> MGSSHHHHHHSSPISPIETVPVKLKPGMDGPKVKQWPLTEEKIKALVEICTEMEKEGKISKIGPENPYNTPVFAIKKKDSTKWRKLVDFRELNKRTQDFWEVQLGIPHPAGLKKKKSVTVLDVGDAYFSVPLDEDFRKYTAFTIPSINNETPGIRYQYNVLPQGWKGSPAIFQSSMTKILEPFRKQNPDIVIYQYMDDLYVGSDLEIGQHRTKIEELRQHLLRWGLTTPDKKHQKEPPFLWMGYELHPDKWTVQPIVLPEKDSWTVNDICKLVGKLNWASQIYPGIKVRQLSKLLRGTKALTEVIPLTEEAELELAENREILKEPVHGVYYDPSKDLIAEIQKQGQGQWTYQIYQEPFKNLKTGKYARMRGAHTNDVKQLTEAVQKITTESIVIWGKTPKFKLPIQKETWETWWTEYWQATWIPEWEFVNTPPLVKLWYQLEKEPIVGAETFYVDGAANRETKLGKAGYVTNRGRQKVVTLTDTTNQKTELQAIYLALQDSGLEVNIVTDSQYALGIIQAQPDQSESELVNQIIEQLIKKEKVYLAWVPAHKGIGGNEQVDKLVSAGIRKVL;> PISPIETVPVKLKPGMDGPKVKQWPLTEEKIKALVEICTEMEKEGKISKIGPENPYNTPVFAIKKKDSTKWRKLVDFRELNKRTQDFWEVQLGIPHPAGLKKKKSVTVLDVGDAYFSVPLDEDFRKYTAFTIPSINNETPGIRYQYNVLPQGWKGSPAIFQSSMTKILEPFRKQNPDIVIYQYMDDLYVGSDLEIGQHRTKIEELRQHLLRWGLTTPDKKHQKEPPFLWMGYELHPDKWTVQPIVLPEKDSWTVNDIQKLVGKLNWASQIYPGIKVRQLSKLLRGTKALTEVIPLTEEAELELAENREILKEPVHGVYYDPSKDLIAEIQKQGQGQWTYQIYQEPFKNLKTGKYARMRGAHTNDVKQLTEAVQKITTESIVIWGKTPKFKLPIQKETWETWWTEYWQATWIPEWEFVNTPPLVKLWYQLEKEPIVGAETF

NRTIs mimic natural deoxynucleosides or deoxynucleotides and target the reverse transcriptase (RT) enzyme. RT incorporates active metabolites of NRTIs into the growing DNA chain which act as chain terminators due to their lack of 3ʹ-OH. M184 is part of the conserved active site YMDD motif found in several viral polymerases, including HIV-1 RT and HBV polymerase. Herein, using the same DNA construct, we report the pre-steady-state kinetic analysis with WT RT and M184V to determine the incorporation efficiency of both (+)- and (−)-enantiomers of FTC-TP and 3TC-TP compared to dCTP in addition to crystal structures of WT RT in complex with dsDNA (RT–DNA) bound to either, (−)-FTC-TP, (−)-3TC-TP, (+)-FTC-TP, or dCTP.

In order to compare how the cytosine based NRTIs bind in relation to the natural substrate, the structure of the ternary complex of RT, DNA and dCTP (RT–DNA•dCTP) was determined. The triphosphates interact with a Mg2+ ion with octahedral coordination, as well as R72, K65, and K220. To further help position the phosphates, dCTP forms an intermolecular hydrogen bond (2.8 Å) between its 3ʹ-OH and an oxygen atom from the β-phosphate, thus stabilizing the triphosphate conformation. Comparing the central ring, it is striking that the C1ʹ and C4ʹ have nearly perfect alignment between (−)-FTC-TP and dCTP. The productive triphosphate binding conformation for RT–DNA•(−)-FTC-TP matches well with the triphosphate conformation in RT–DNA•dCTP. For RT–DNA•dCTP, Cγ is positioned closer to the ribose ring. Remarkably, the γC of M184 in the RT–DNA•dCTP structure mimics the branched carbon of valine, suggesting that it has some role in stabilizing dCTP binding. Comparing the position of Cγ in RT–DNA•(−)-FTC-TP to RT–DNA•dCTP, the atom moves 1.8 Å.>[4x]TRTRGYVTTKDGIKWYYEQEGSGPDVVLIPDGLGECQMFDKPMSLIASNGFRVTTFDMPGMSRSSDAPPETYQDITGRKLAGYIITLLDTLDIKIASVWGCASGASTVLALCSDYPERVRNGMPHEVPTENPDILLHIHEVDPATISQEMAANSRAASGNVEAWDALGPEVHARLHDNYPRWAYGYPRTIPPS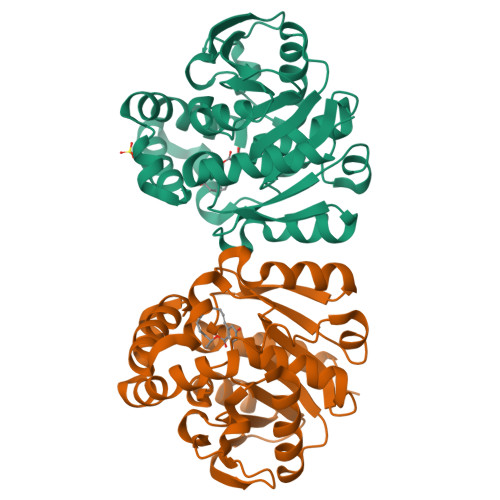APVKTEDLHKVPIDWTVGASTPTKLFFENIVIAAREGINIGTLPGNHFPYVSHPEEFAKYVVETSRKYLK> VGRALPDVRDGLKPVHRRVLYAMNVLGNDWNKAYKKSARVVGDVIGKYHPHGDSAVYDTIVRMAQPFSLRYMLVDGQGNFGSIDGDSAAAMRYTEIRLAKIAHELMADLEKETVDFVDNYDGTEKIPDVMPTKIPNLLVNGSSGIAVGMATNIPPHNLTEVINGCLAYIDDEDISIEGLMEHIPGPDFPTAAIINGRRGIEEAYRTGRGKVYIRARAEVEVDAKTGRETIIVHEIPYQVNKARLIEKIAELVKEKRVEGISALRDESDKDGMRIVIEVKRDAVGEVVLNNLYSQTQLQVSFGIN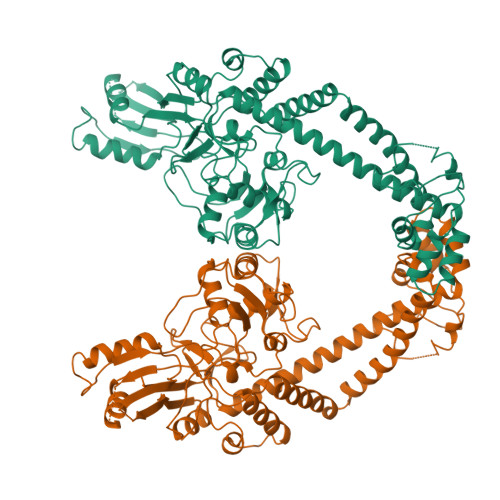MVALHHGQPKIMNLKDIIAAFVRHRREVVTRRTIFELRKARDRAHILEALAVALANIDPIIELIRHAPTPAEAKTALVANPWQLGNVAAMLERAGDDAARPEWLEPEFGVRDGLYYLTEQQAQAILDLRLQKLTGLEHEKLLDEYKELLDQIAELLRILGSADRLMEVIREELELVREQFGDKRRTEIT> MCLKRKAPHLFCFCLWSIFLSFRCFCFRSYAIMLPLLSFPTIQISIFLSFKLPITTFLLSPCFVFVFVFAIRYCGELTLNAQLVLFLLYHCAQTQRGPLKEGEMPICPGLCGELAAVPFRVFLGTLPTLAVEERFLRQLQPVFAWYSSRKRVKEQANEFIEIDLASCDAELLLRYSHIYYVRRQLFDELIERQMTLLDSGKAPKMAEPSLLQCLAGCNMTIADRLQLEIRQLGAAKRAASVPGRRELDPVARLEVYDYACMMRLVEEDAGAVGDAEMKARAYLPREVIESKLGHLTQLLL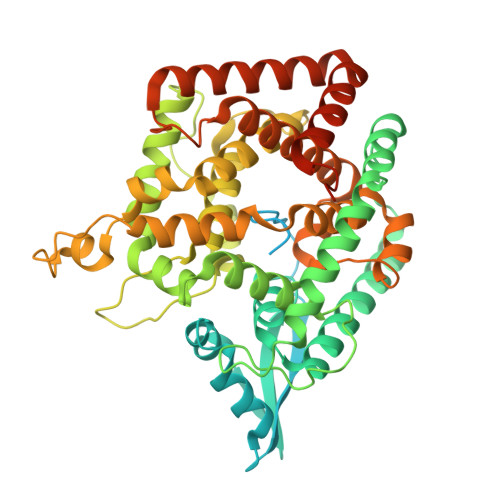GSDARAALDKKDVKLLNRMIPPDYTRVGCVEKLRPFDVTAYFRFYGERINNVKVENYFKRALWGHVYRRFATTPSFLSGVSTYWARHSGLDASFTTTTMPQEVAVAVCDQQIQFPAIKFRAQYVYTSPETARQLWRTDAAVPLMRLFPLMGSRTAEDLAAGVLTDAFWMHLGLSEEENLLQDSLLLKVRRFVDEVGDMYETNIDSVLKRVDDNFKQVVPQLKAEDLQVDAPLQDGEGEDTVRETVAA>[3x]MDSPTQIFEHVFLGSEWNASNLEDLQNRGVRYILNVTREIDNFFPGVFEYHNIRVYDEEATDLLAYWNDTYKFISKAKKHGSKCLVHSKMGVSRSASTVIAYAMKEYGWNL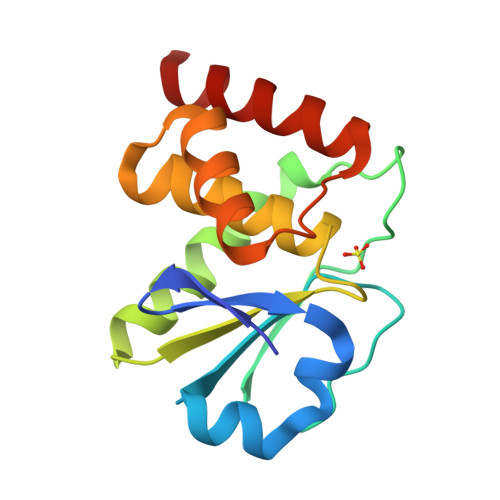DRAYDYVKERRTVTKPNPSFMRQLEEYQGILLAR>GFKQDIATIRGDLRTYAQDIFLAFLNKYPDERRYFKNYVGKSDQEL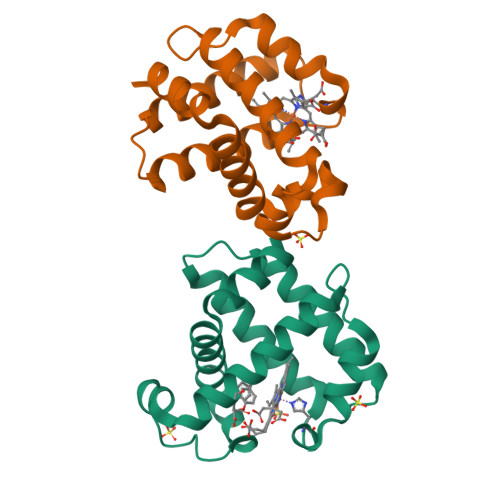KSMAKFGDDTEKVFNLMMEVADRATDCVPLASDANTLVQMKQHSSLTTGNFEKLFVALVEYMRASGQSFDSQSWDRFGKNLVSALSSAGMK[2x]>[4x]MKLERVTVKNFRSHSDTVVEFKEGINLIIGQNGSGKSSLLDAILVGLYWPLRIKDIKKDEFTKV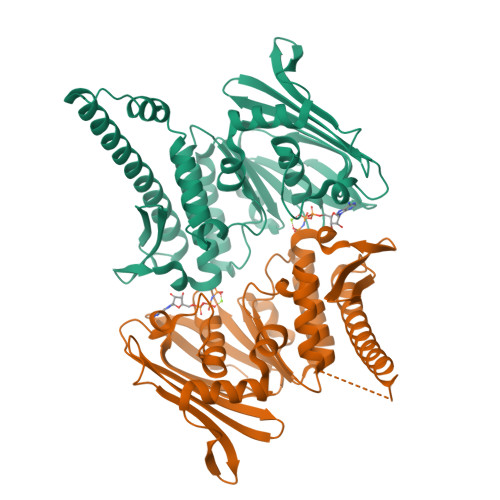GARDTYIDLIFEKDGTKYRITRRFLKGYSSGEIHAMKRLVGNEWKHVTEPSSKAISAFMEKLIPYNIFLNAIYIRQGQIDAILESDEAREKVVREVLNLDKFETAYKKLSELKGGSGGTEELIEKVKKYKALAREAALSKIGELASEIFAEFTEGKYSEVVVRAEENKVRLFVVWEGKERPLTFLSGGERIALGLAFRLAMSLYLAGEISLLILDEPTPYLDEERRRKLITIMERYLKKIPQVILVSHDEELKDAADHVIRISLENGSSKVEVVS> MRGSHHHHHHGSEEASSTGRNFNVEKINGEWHTIILASDKREKIEDNGNFRLFLEQIHVLEKSLVLKFHTVRDEECSELSMVADKTEKA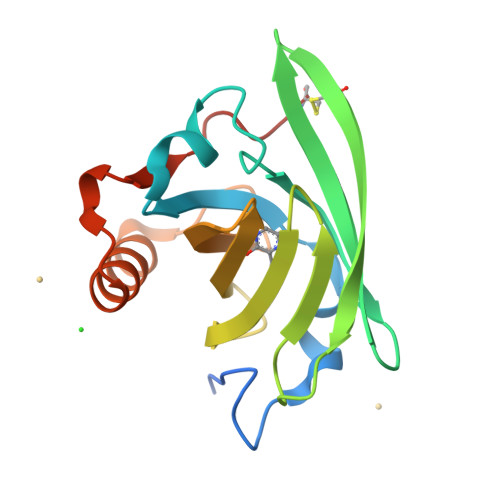GEYSVTYDGFNTFTIPKTDYDNFLMAHLINEKDGETFQLMGLFGREPDLSSDIKERFAQLCEEHGILRENIIDLSNANRCLQARE Sm and Sm-like (Lsm) proteins have been found in all three kingdoms of life: bacteria, archaea and eukaryotes. They are essential parts of ribonucleoprotein (RNP) complexes and are actively involved in various steps of RNA metabolism including pre-mRNA splicing, mRNA degradation, telomere replication, histone formation and translational control. Members of this protein family are characterized by two closely spaced, conserved Sm motifs 1 and 2, which adopt a conserved Sm fold that consists of an N-terminal α helix followed by a twisted five-stranded β sheet. A common characteristic of Sm/Lsm proteins is their tendency to form a hepta- or hexameric ring structure.

Attempts of crystallization of full length SpLsm4 failed due to the poor solubility and low yield of the full length protein. The structure of SpLsm4N was also determined by the SAD method using the data obtained from a SeMet derivative crystal. The structure has been refined at a resolution of 2.2 Å to an R factor of 23.7% and Rfree of 25.2% with good geometry. The final model covers residues 12–71 of every molecule in the AU. Residues 1–11 and 72–91 are not visible in the electron density map and assumed to be disordered. Consistent with this notion, our structures showed that a possible arrangement of a dimer of heptamers, a trimer and a hexamer for SpLsm3, SpLsm4N and SpLsm5/6/7, respectively, in the crystal lattice. Surface plasmon resonance analysis in combination with fluorescence anisotropy analysis revealed that SpLsm2/3, and SpLsm5/6/7 bound to oligo(U) whereas no binding of oligo(U) was observed for SpLsm3 and SpLsm4N.

>[24x]MGSSHHHHHHSQDPMLPLTLLNATQGRPILVELKNGETFNGHLENCDNYMNLTLREVIRTMPDGDKFFRLPECYIRGNNIKYLRIQDEVLSQVAKQQAQQRENRG> MPPQLHNGLDFSAKVIQGSLDSLPQEVRKFVEGNAQLCQPEYIHICDGSEEEYGRLLAHMQEEGVIRKLKKYDNCWLALTDPRDVARIESKTVIITQEQRDTVPIPKSGQSQLGRWMSEEDFEKAFNARFPGCMKGRTMYVIPFSMGPLGSPLAKIGIELTDSPYVVASMRIMTRMGTSVLEALGDGEFIKCLHSVGCPLPLKKPLVNNWACNPELTLIAHLPDRREIISFGSGYGGNSLLGKKCFALRIASRLAKEEGWLAEHMLILGITNPEGKKKYLAAAFPSACGKTNLAMMNPTLPGWKVECVGDDIAWMKFDAQGNLRAINPENGFFGVAPGTSVKTNPNAIKTIQKNTIFTNV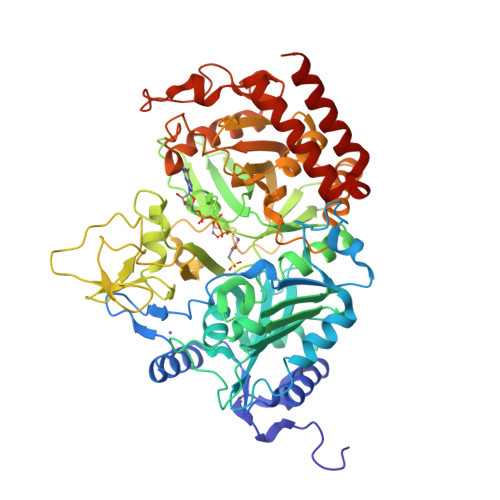AETSDGGVYWEGIDEPLAPGVTITSWKNKEWRPQDEEPCAHPNSRFCTPASQCPIIDPAWESPEGVPIEGIIFGGRRPAGVPLVYEALSWQHGVFVGAAMRSEGIMHDPFAMRPFFGYNFGKYLAHWLSMAHRPAAKLPKIFHVNWFRKDKNGKFLWPGFGENSRVLEWMFGRIEGEDSAKLTPIGYVPKEDALNLKGLGDVNVEELFGISKEFWEKEVEEIDKYLEDQVNADLPYEIERELRALKQRISQM DyPs (dye-decolorizing peroxidases) (EC 1.11.1.19) represent a new family of haem peroxidases widespread in bacteria, archaea, fungi and other micro-organisms. In the present study, we expressed A. auricula-judae DyP in E. coli, solved the crystal structure of the recombinant enzyme and several site-directed variants, and used PELE (Protein Energy Landscape Exploration) to describe the binding of its typical substrate RB19. The DyP structure is formed by two domains, each of them including an antiparallel four-stranded large β-sheet and two or three helices resulting in a ferredoxin-like fold (plus two additional β-strands). In spite of the obvious similarity between the two domains, only the C-terminal domain harbours a haem cofactor.

His-304 (Nε) acts as the fifth ligand of the haem iron, with Asp-395 at 2.66 Å. To identify the possible substrate binding site(s) in A. auricula-judae DyP, we performed 160 PELE non-biased simulations, where the typical DyP substrate RB19 was free to explore the structure of the recombinant enzyme. These simulations show that RB19 encounters several favourable docking positions on the protein surface, with local minima close to Trp-105, Tyr-147/Tyr-337, Trp-207, Tyr-285 and Trp-377 sites, as well as in the haem channel entrance. There is a clear preference for Trp-377 to be oxidized over Trp-105, Tyr-285 and Tyr-337. Finally, using QM/MM methods, we were able to map the important residues along the LRET pathway from WT DyP Trp-377 to the haem. This pathway would include a first 3.0 Å electron transfer between the Trp-377 side chain and the Pro-310/Arg-309 backbone, and a second one (2.9 Å) between the Arg-309 and Arg-306 carbonyls, followed by the Arg-306 to His-304 backbone to reach the haem iron (at only 2.2 Å from the His-304 side chain). The EPR spectrum of the WT DyP resting state (top) shows a ferric species prevalently in its axial high spin state (g⊥≈ 6 and g∥=2.0). After adding 10 eq. of H2O2, a strong decrease in the ferric signal, and appearance of an intense protein radical signal are evident (bottom) (the electronic absorption spectra of WT DyP, and the EPR and electronic absorption spectra of the D168N and R332L variants are described in the Supplementary Results and Supplementary Figures S4 and S5 respectively). The yield of the radical observed in the spectrum of the H2O2-activated WT DyP is estimated as 0.58 spin/haem. Simultaneously, a mixed tryptophanyl/tyrosyl radical was detected by EPR spectroscopy of the H2O2-activated WT (wild-type) DyP.

>MATSLNTIDIQGDILVGMHKQKQLFYFFAINDPATFKTHLASDIAPVVASVTQLSNVATQPLVALNIAFSNTGLLALGVTDNLGDSLFANGQAKDATSFKESTSSWVPQFAGTGIHGVIILASDTTDLIDQQVASIESTFGSSISKLYSLSASIRPGNEAGHEMFGFLDGIAQPAINGFNTPLPGQNIVDAGVIITGATNDPITRPSWAVGGSFLAFRQLEQLVPEFNKYLLDNAPAGSGSLQARADLLGARMVGRWKSGAPIDLTPTADDPALGADAQRNNNFTYSHAGFDLGSDQSHCPFSAHIRKTRPRADLGGSLTPPNLSAGANSIMRSGIPYGPEVTSAESASNTTTQERGLAFVAYQAQLSQGFHFLQQTWADNANFPPGKTPATVGLDPIIGQNNGQPRVVNGLLPSNSSASLSIPQFVVSHGGEYFFSPPISAIGGRLSA[4x]> MSSLLDIIYQLRQVPR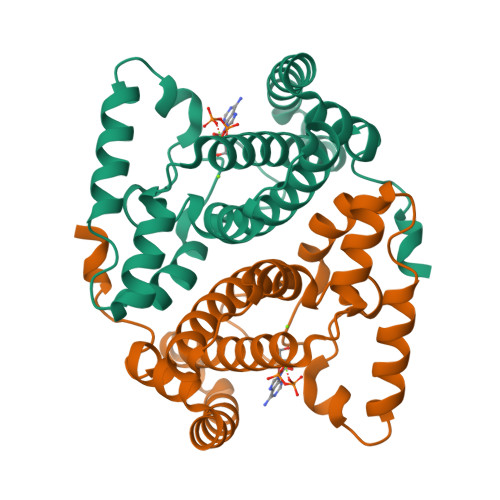WDGSFQFEKEDVSQHSFSVIAISHILCELKETLEGKKINKEKLLLYALYHDVTEVVSTHIISPVKKNSILKDPFNAFREQIKNSLFDNLPITLSDTLSTILNNNDLEIQEIVEHADHVDAYCKSCIEVHRGNKDFISIQRSLGDKLDNLTKEYPYLKEFQNLFLKDFPLENKNYRYLN>MSKTVILSAARTPVGKFGGSLKDVKATELGGIAIKAALERANVAASDVEEVIFGTVIQGGQGQIPSRQAARAAGIPWEVQTETVNKVCASGLRAVTLADQIIRTGDQSLIV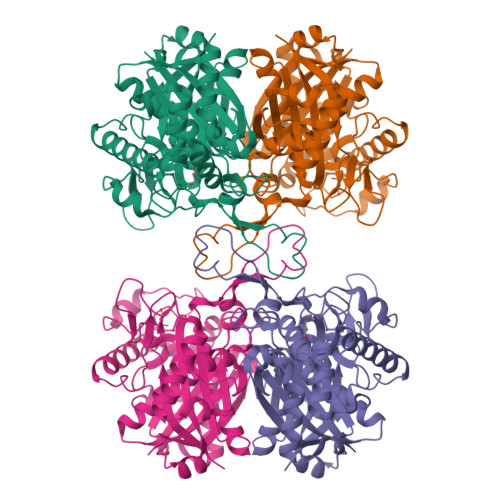AGGMESMSNSPYILRGARWGYRMGNNEVIDLNVADGLTCAFSGTHMGVYGGEVAKEDGISREAQDEWAYRSHQRAVSAHKEGRFEEEIVPVTIPQRKGDPIVVAKDEAPREDTTIEKLAKLKPVFDKTATVTAGNAPGLNDGGAALVLMSEDRAKQEGRKPLATILAHTAIAVESKDFPRTPGYAINALLEKTGKTIEDIDLFEINEAFAAVAIASTEIAGIDPEKLNVNGGAVAMGHPIGASGARIIVTLIHALKQRGGGIGIASICSGGGQGDAVMIEVHLEHHHHHH[2x]> GSHMASMRVVKEL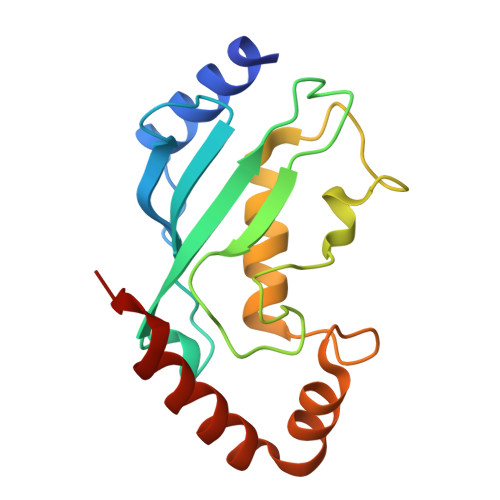EDLQKKPPPYLRNLSSDDANVLVWHALLLPDQPPYHLKAFNLRISFPPEYPFKPPMIKFTTKIYHPNVDENGQICLPIISSENWKPCTKTCQVLEALNVLVNRPNIREPLRMDLADLLTQNPELFRKNAEEFTLRFGVDRPS>MSTGTSNLVAVEPGAIREDTPPGSVIQYSDYELDHSSPFAGGVAWIEGEFLPAEDAKISIFDTGFGHSDLTYTVAHVWHGNIFRLGDHLDRLLDGARKLRLDAGYTKDELADITKQCVSMSQLRESFVNLTVTRGYGKRRGEKDLSKLTHQVYIYAIPYLWAFPPAEQIFGTTAIVPRHVRRAGRNTVDPTIKNYQWGDLTAASFEAKDRGARTAILLDSDNCVAEGPGFNVCIVKDGKLASPSRNALPGITRKTVFEIADQMGIEATLRDVTSHELYDADELMAVTTAGGVTPINSLDGEAIGNGAPGPMTVAIRDRFWALMDEPGPL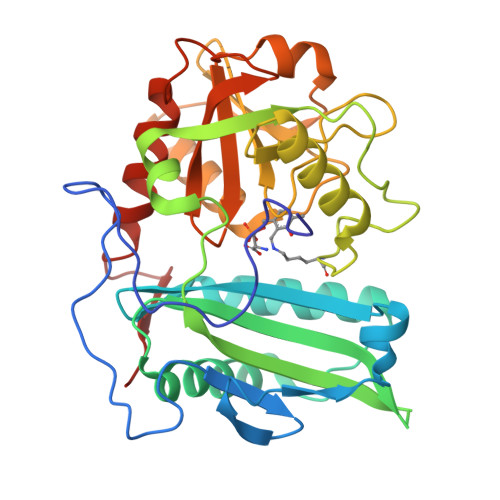IEAIEY[4x]> ALVVTDPLTRTECSACHMAYPAALLPARSWTALMADLPNHFGEDASLDEASRGQIESYLVANAADSSGAGRALRGLVQTDTPLRISELPWFKRKHADEVSP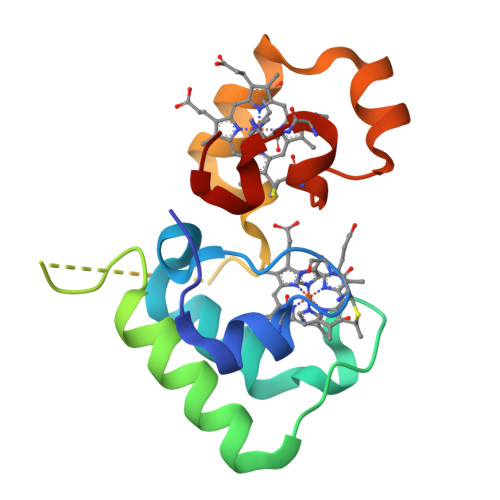RMLEKARSMSNCAACHTGAERGLF>PTSDDIFEREYKYGAHNYHPLPVALERGKGIYLWDVEGRKYFDFLSSYSAVNQGHCHPKIVNALKSQVDKLTLTSRAFYNNVLGEYEEYITKLFNYHKVLPMNTGVEAGETACKLARKWGYTVKGIQKYKAKIVFAAGNFWGRTLSAISSSTDPTSYDGFGPFMPGFDIIPYNDLPALERALQDPNVAAFMVEPIQGEAGVVVPDPGYLMGVRELCTRHQVLFIADEIQTGLARTGRWLAVDYENVRPDIVLLGKALSGGLYPVSAVLCDDDIMLTIKPGEHGSTYGGNPLGCRVAIAAL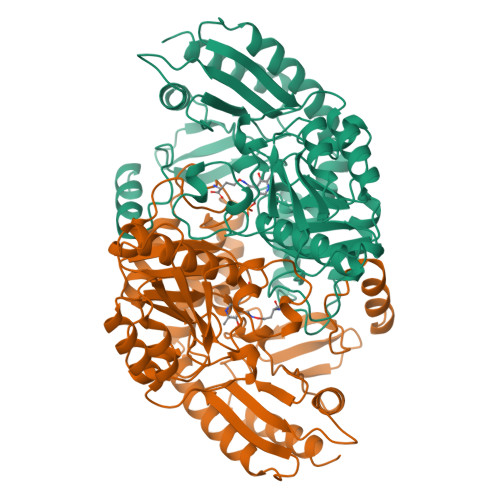EVLEEENLAENADKLGIILRNELMKLPSDVVTAVRGKGLLNAIVIKETKDWDAWKVCLRLRDNGLLAKPTHGDIIRFAPPLVIKEDELRESIEIINKTILSF[3x]>GSHMLDHVRVGVVITDPALEDNPIVYVNQGFVQMTGYETEEILGKNCRFLQG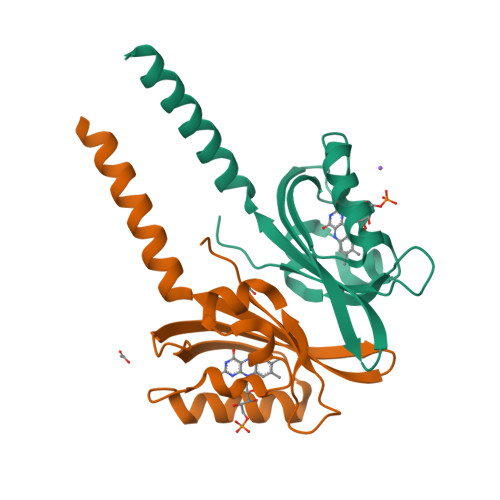KHTDPAEVDNIRTALQNKEPVTVQIQNYKKDGTMFWNELNIDPMEIEDKTYFVGIQNDITKQKEYEKLLEDSLTEITALS[2x]>[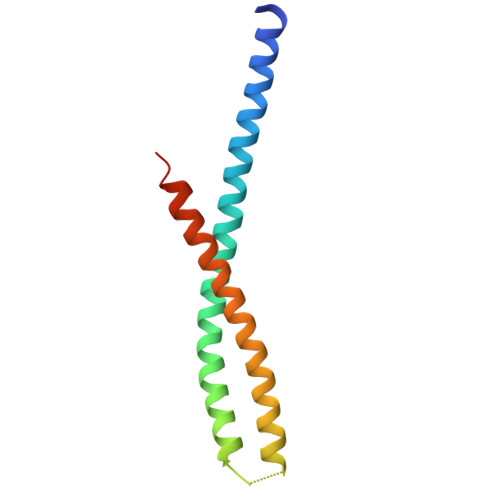2x]ATDAASLVGELQALDAEYQNLANQEEARFNEERAQADAARQALAQNEQVYNELSQRAQRLQAEANGGGGKSQYQELASKYEDALKKLEAEMEQQKAVISDFEKIQALRAGNLEHHHHHH2-{[(carbamoylsulfanyl)acetyl]amino}benzoic acid | C10 H10 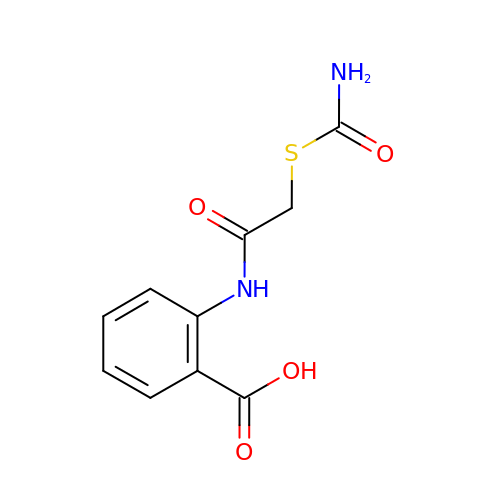N2 O4 S | NWUAPELPCMQTDN-UHFFFAOYSA-N>[5x]MLVSVYLALLVACVGQAHSQANLMRLKSDLFNRSPMYPGPTKDDPLTVTLGFTLQDIVKVDS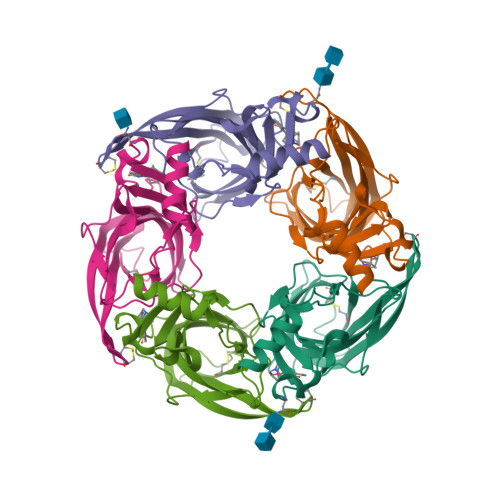STNEVDLVYYEQQRWKLNSLMWDPNEYGNITDFRTSAADIWTPDITAYSSTRPVQVLSPQIAVVTHDGSVMFIPAQRLSFMCDPTGVDSEEGVTCAVKFGSWVYSGFEIDLKTDTDQVDLSSYYASSKYEILSATQTRQVQHYSCCPEPYIDVNLVVKFRERRAGNGFFRNLFDENLYFQGHHHHHH CYCLO-(L-HISTIDINE-L-PROLINE) INHIBITOR | C11 H14 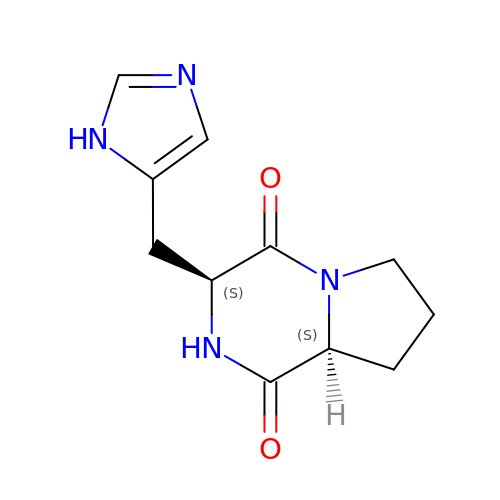N4 O2 | NAKUGCPAQTUSBE-IUCAKERBSA-N>[2x]GAMNAQAEEFKKYLETNGIKPKQFHKKELIFNQWDPQEYCIFLYDGITKLTSISENGTIMNLQYYKGAFVIMSGFIDTETSVGYYNLEVISEQATAYVIKINELKELLSKNLTHFFY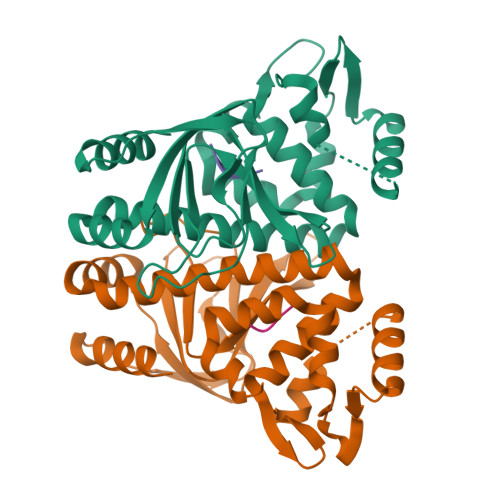VFQTLQKQVSYSLAKFNDFSINGKLGSICGQLLILTYVYGKETPDGIKITLDNLTMQELGYSSGIAHSSAVSRIISKLKQEKVIVYKNSCFYVQNLDYLKRYAPKLDEWFYLACPATWGKLN;>RGLL[2x]> EES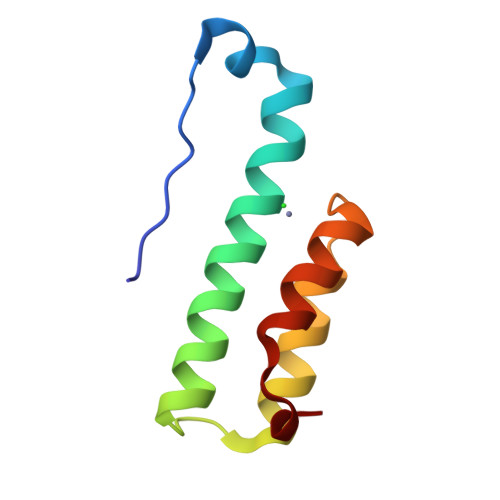ISLTFRNMNDFTPEQVARQIPRLKAMLAMRSLLRDLKANLLDNVTFRKELEKILRDPALSQTLRDELRALVPEKAW N-[2-(2,4-dimethylphenyl)-4,6-dihydrothieno[3,4-c]pyrazol-3-yl]-4-(phenylcarbonyl)benzamide 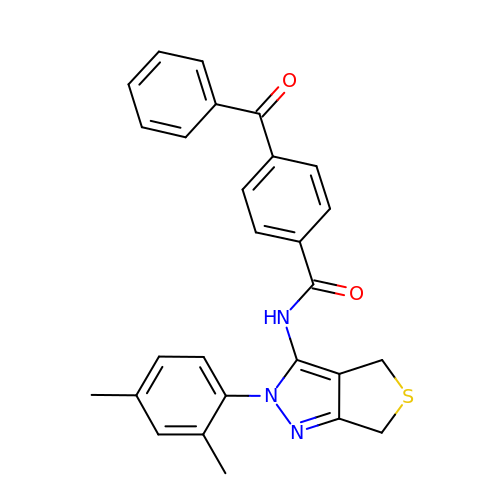| C27 H23 N3 O2 S | XTWGDUKLCYCIKR-UHFFFAOYSA-N N-[(3S)-2-oxotetrahydrofuran-3-yl]hexanamide | C10 H17 N O3 | 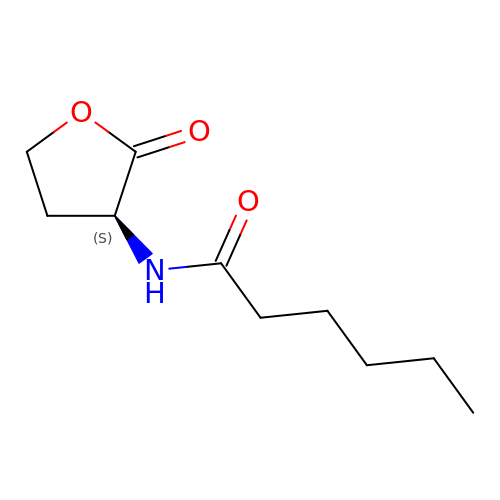ZJFKKPDLNLCPNP-QMMMGPOBSA-N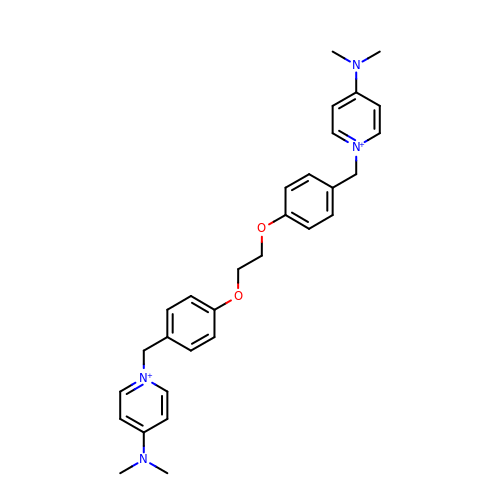1-[[4-[2-[4-[[4-(dimethylamino)pyridin-1-yl]methyl]phenoxy]ethoxy]phenyl]methyl]-N,N-dimethyl-pyridin-4-amine | C30 H36 N4 O2 | SBSYTSUJNSFXCL-UHFFFAOYSA-N> GATVAPSSRRDFTFDLYRALASAAPSQNIFFSPVSISMSLAMLSLGAGSSTKMQILEGLGLNLQKSSEKELHRGFQQLLQELNQPRDGFQLSLGNALFTDLVVDLQDTFVSAMKTLYLADTFPTNFRDSAGAMKQINDYVAKQTKGKIVDLLKNLDSNAVVIMVNYIFFKAKWETSFNHKGTQEQDFYVTSETVVRVPMMSREDQYHYLLDRNLSCRVVGVPYQGNATALFILPSEGKMQQVENGLSEKTLRKWLKMFKKRQLE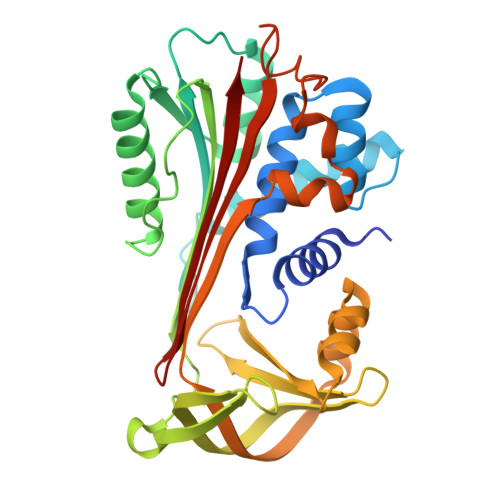LYLPKFSIEGSYQLEKVLPSLGISNVFTSHADLSGISNHSNIQVSEMVHKAVVEVDESGTRAAAATGTIFTF>[2x]MAHHHHHHMSAQVMLEEMARKYAINAVKAD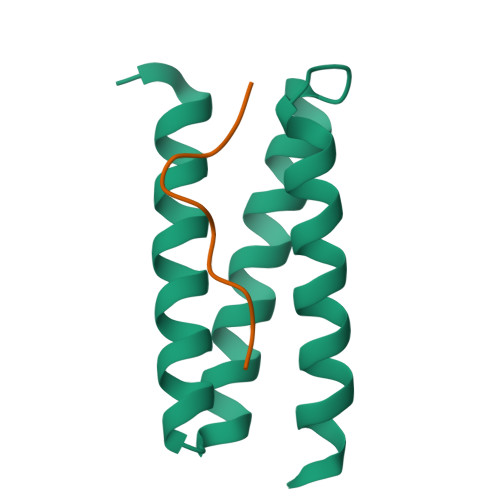KEGNAEEAITNYKKAIEVLAQLVSLYRDGSTAAIYEQMINEYKRRIEVLKELI;>[2x]VRELLPELPHPPSE> MAKSSKGAGKSLVRANLAIHEPPTGKSTSPGGLIKRFPFEFNPAQLSISQRSQWKATPTAAVRKAAKPQFMGAEPREMTLEIFLDSSMKPGGNTVMKKVESLLICCEVTAKSLAAKQPSPPWVIFEWGSFSTARFNAY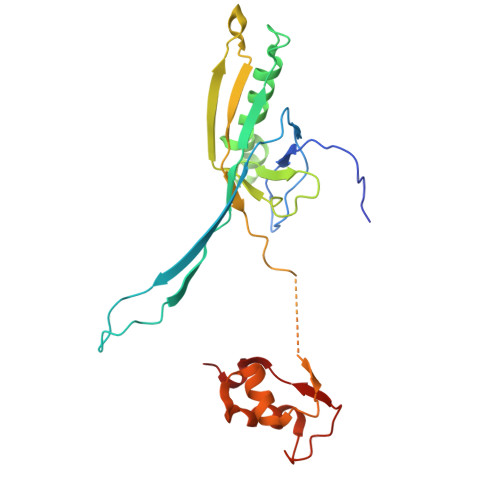VASIETQYTLFGTAGVPIRATCQMGLVEIPGPTPNQNPTSGALTAQRVHRVVAGDSLQSLAWSEYGSANAWRVIAEANGIDDPSHLPTGTELILPATEEVPH> GPHMKTHIDDYSTWDIVKATQYGIYERCRELVEAGYDVRQPDKANVTLLHWAAINNRIDLVKYYISKGAIVDQLGGDLNSTPLHWATRQGHLSMVVQLMKYGADPSLIDGEGCSCIHLAAQFGHTSIVAYLIAKGQDVDMMDQNGMTPLMWAAYRTHSVDPTRLLLTFNVSVNLGDKYHKNTALHWAVLAGNTTVISLLLEA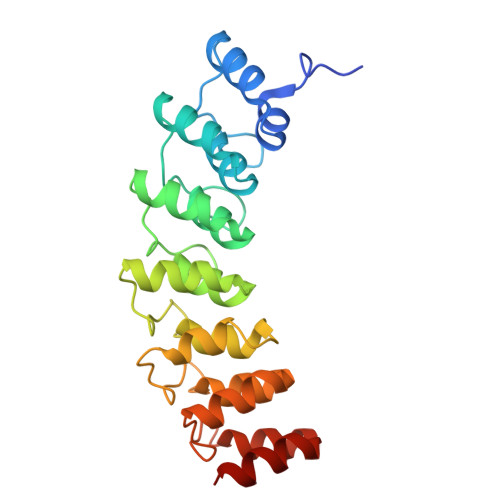GANVDAQNIKGESALDLAKQRKNVWMINHLQEARQAK> MYYESLTKQYPVSKTIRNELIPIGKTLDNIRQNNILESDVKRKQNYEHVKGILDEYHKQLINEALDNCTLPSLKIAAEIYLKNQKEVSDREDFNKTQDLLRKEVVEKLKAHENFTKIGKKDILDLLEKLPSISEDDYNALESFRNFYTYFTSYNKVRENLYSDKEKSSTVAYRLINENFPKFLDNVKSYRFVKTAGILADGLGEEEQDSLFIVETFNKTLTQDGIDTYNSQVGKINSSINLYNQKNQKANGFRKIPKMKMLYKQILSDREESFIDEFQSDEVLIDNVESYGSVLIESLKSSKVSAFFDALRESKGKNVYVKNDLAKTAMSNIVFENWRTFDDLLNQEYDLANENKKKDDKYFEKRQKELKKNKSYSLEHLCNLSEDSCNLIENYIHQISDDIENIIINNETFLRIVINEHDRSRKLAKNRKAVKAIKDFLDSIKVLERELKLINSSGQELEKDLIVYSAHEELLVELKQVDSLYNMTRNYLTKKPFSTEKVKLNFNRSTLLNGWDRNKETDNLGVLLLKDGKYYLGIMNTSANKAFVNPPVAKTEKVFKKVDYKLLPVPNQMLPKVFFAKSNIDFYNPSSEIYSNYKKGTHKKGNMFSLEDCHNLIDFFKESISKHEDWSKFGFKFSDTASYNDISEFYREVEKQGYKLTYTDIDETYINDLIERNELYLF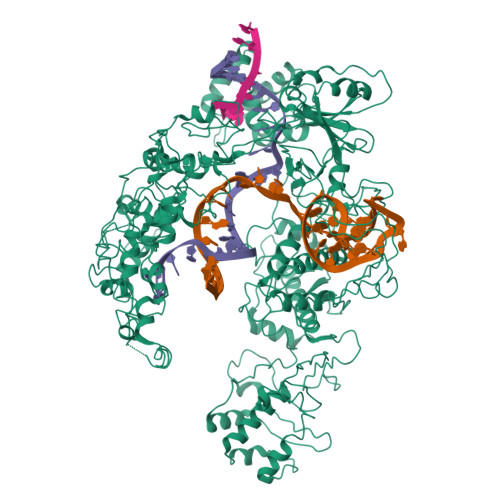QIYNKDFSMYSKGKLNLHTLYFMMLFDQRNIDDVVYKLNGEAEVFYRPASISEDELIIHKAGEEIKNKNPNRARTKETSTFSYDIVKDKRYSKDKFTLHIPITMNFGVDEVKRFNDAVNSAIRIDENVNVIGIDRGERNLLYVVVIDSKGNILEQISLNSIINKEYDIETDYHALLDEREGGRDKARKDWNTVENIRDLKAGYLSQVVNVVAKLVLKYNAIICLEDLNFGFKRGRQKVEKQVYQKFEKMLIDKLNYLVIDKSREQTSPKELGGALNALQLTSKFKSFKELGKQSGVIYYVPAYLTSKIDPTTGFANLFYMKCENVEKSKRFFDGFDFIRFNALENVFEFGFDYRSFTQRACGINSKWTVCTNGERIIKYRNPDKNNMFDEKVVVVTDEMKNLFEQYKIPYEDGRNVKDMIISNEEAEFYRRLYRLLQQTLQMRNSTSDGTRDYIISPVKNKREAYFNSELSDGSVPKDADANGAYNIARKGLWVLEQIRQKSEGEKINLAMTNAEWLEYAQTHLL> MNHKVHMASQPNSSAKKKEEKGKNIQVVVRCRPFNLAERKASAHSIVECDPVRKEVSVRTGGLADKSSRKTYTFDMVFGASTKQIDVYRSVVCPILDEVIMGYNCTIFAYGQTGTGKTFTMEGERSPNEEYTWEEDPLAGIIPRTLHQIFEKLTDNGTEFSVKVSLLEIYNEELFDLLNPSSDVSERLQMFDDPRNKRGVIIKGLEEIT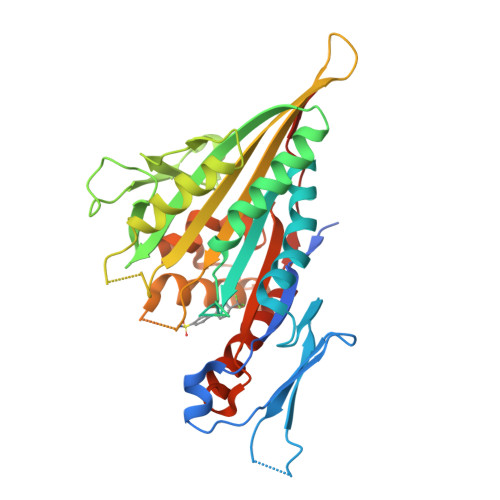VHNKDEVYQILEKGAAKRTTAATLMNAYSSRSHSVFSVTIHMKETTIDGEELVKIGKLNLVDLAGSENIGRSGAVDKRAREAGNINQSLLTLGRVITALVERTPHVPYRESKLTRILQDSLGGRTRTSIIATISPASLNLEETLSTLEYAHRAKNILNKPEVNQKLQHHHHHH> MIRRYLYTFLLVMTLAGCKDKDLLKGLDQEQANEVIAVLQMHNIEANKIDSGKLGYSITVAEPDFTAAVYWIKTYQLPPRPRVEIAQMFPADSLVSSPRAEKARLYSAIEQRLEQSLQTMEGVLSARVHISYDIDAGENGRPPKPVHLSALAVYERGSPLAHQISDIKRFLKNSFADVDYDNISVVLSERSDAQLQAPGTPVKRNSFATSWIVLIILLSVMSAGFGVWYYKN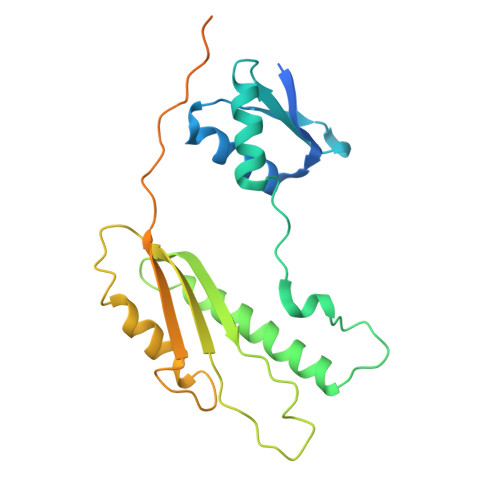HYARNKKGITADDKAKSSNE>[4x]SNARVHRVTRSFVGNREIGQITLKKDQ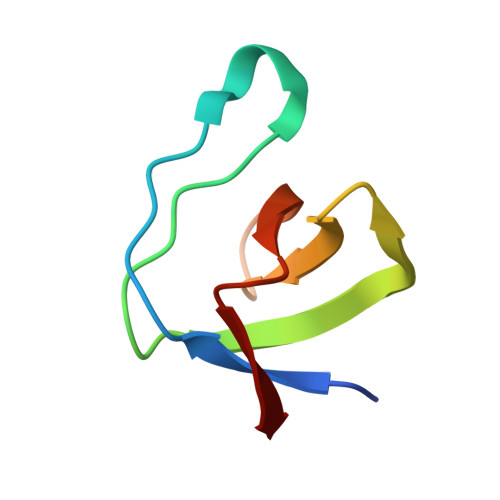IVVQKGDEAGGYVKVYTGRKVGLFPTDFLEEI3-{2,6,8-TRIOXO-9-[(2R,3R,4R)-2,3,4,5-TETRAHYDROXYPENTYL]-1,2,3,6,8,9-HEXAHYDRO-7H-PURIN-7-YL}PROPYL DIHYDROGEN PHOSPHATE | C13 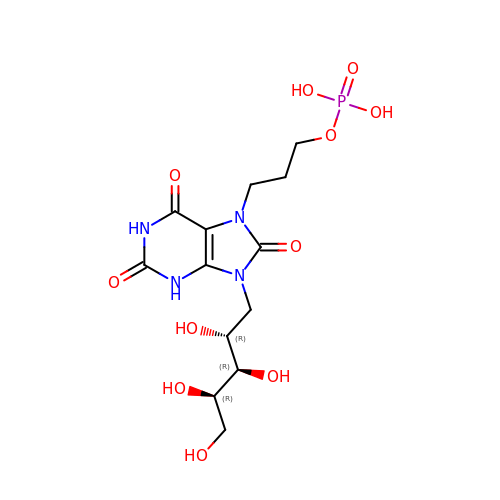H21 N4 O11 P | KPHFGOGGKPGLTM-ZXFLCMHBSA-N> QTTPNSEGWHDGYYYSWWSDGGAQATYTNLEGGTYEISWGDGGNLVGGKGWNPGLNARAIHFEGVYQPNGNSYLAVYGWTRNPLVEYYIVENFGTYDPSSGATDLGTVECDGSIYRLGKTTRVNAPSIDGTQTFDQYWSVRQDKRTSGTVQTG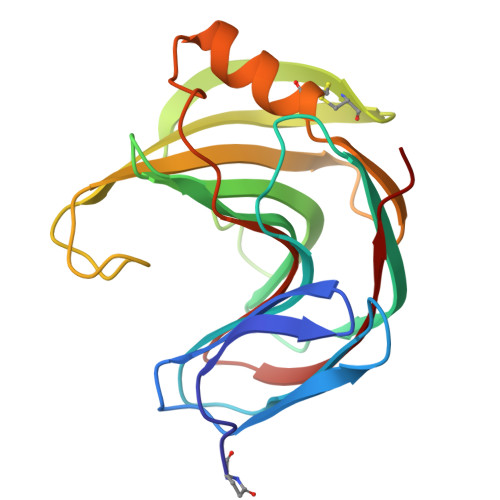CHFDAWARAGLNVNGDHYYQIVATEGYFSSGYARITVADVG> CGCGA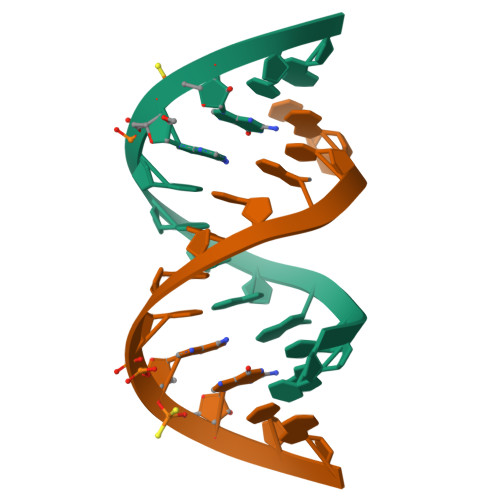AUUAXCG>VNNTIVVSIGQAGNQIAASFWKTVCLEHGIDPLTGQTAPGVAPRGNWSSFFSKLGESSSGSYVPRAIMVDLEPSVIDNVKATSGSLFNPANLISRTEGAGGNFAVGYLGAGREVLPEVMSRLDYEIDKCDNVGGIIVLHAIGGGTGSGFGALLIESLKEKYGEIPVLSCAVLPSPQVSSVVTEPYNTVFALNTLRRSADACLIFDNEALFDLAHRKWNIESPTVDDLNLLITEALAGITASMRFSGFLTVEITLRELLTNLVPQPSLHFLMCAFAPLTPPDRSKFEELGIEEMIKSLFDNGSVFAACSPMEGRFLSTAVLYRGIMEDKPLADAALAAMREKLPLTYWIPTAFKIGYVEQPGISHRKSMVLLANNTEIARVLDRICHNFDKLWQRKAFANWYLNEGMSEEQINVLRASAQELVQSYQVAEESGA[8x];>[8x]VREILSIHVGQCGNQIADSFWRLALREHGLTEAGTLKEGSNAAANSNMEVFFHKVRDGKYVPRAVLVDLEPGVIARIEGGDMSQLFDESSIVRKIPGAANNWARGYNVEGEKVIDQIMNVIDSAVEKTKGLQGFLMTHSIGGGSGSGLGSLILERLRQAYPKKRIFTFSVVPSPLISDSAVEPYNAILTLQRILDNADGAVLLDNEALFRIAKAKLNRSPNYMDLNNIIALIVSSVTASLRFPGKLNTDLSEFVTNLVPFPGNHFLTASFAPMRGAGQEGQVRTNFPDLARETFAQDNFTAAIDWQQGVYLAASALFRGDVKAKDVDENMATIRKSLNYASYMPASGGLKLGYAETAPEGFASSGLALVNHTGIAAVFERLIAQFDIMFDNHAYTHWYENAGVSRDMMAKARNQIATLAQSYRDAS;>DTALERQIASASRSVEEARRLAYHDPIRVG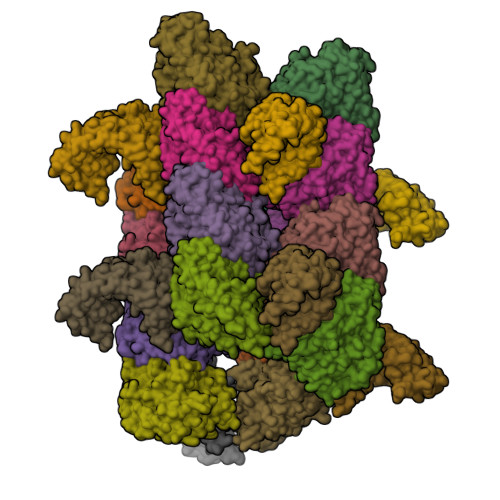ALVEQISVLADLRQKEGDFRKAESLYREALFRAQELRKQDPDLLTGIYSLLAHLYDRWGRMDKAAEFYELALKISAENGLEESDKVATIKNNLAMIFKQLRKFERAEGYYCEALETFQRLDGEQSARVASVYNNLGVLYYSHMDVDRAQVMHERALAIRQNLHEGQMDPADLSQTFINLGAVYKAAGDFQKAEACVDRAKRIRAAMNG[8x]>[4x]GHAKSVPSR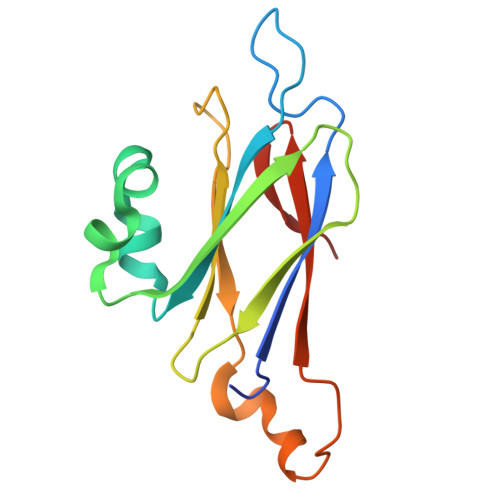YSLVFDADRQVNAAAGAQPAPIKIRVLLLRSDAEFMDADFFSLQNDAKSVLGNSLLDSDQFFLTPGQTGKKLGGQSALDARYIGVIAEYQNLDGKTWRISLPLPEPTETNFYKVWQFSPDELEAHIVAGVSGLRPVKKVD> MSEVEDTLNRIKTHKTVLGYLIVNSEGGVVRGAFKDEEESKNIANSIPLLTKKARSVVRDLDPTNDLVFLRIQTKLNEIMVAPDDEFSLIVIQTKGEKR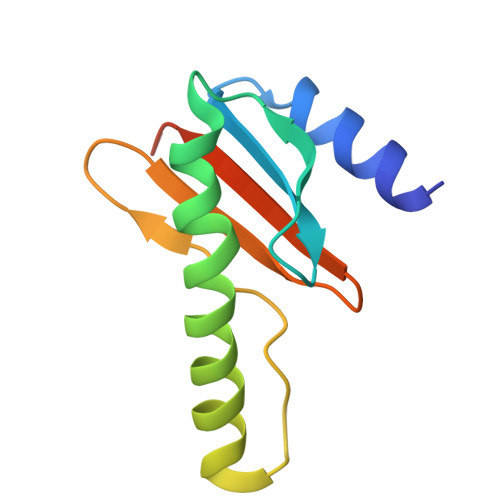DEND> AIPSSLSINWNNYATGAYSSGNAASDFGNAGGWNQSRSYISDGTLRVTLLKNALSGAGGLISNIDVSDGTEYELDYDVRFHSQFDWSRGGKVGFGFSIGEGNTGGDPGWDGNGGTLRMMWYQTDAGRVFFQPYIYHKDQPGQY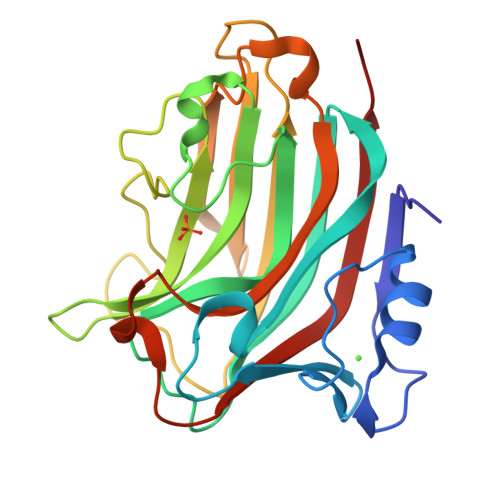GDTFGKSYPSSGSITKGTTYHVHVYIKSNTGSNRDGRAQIIINGTTVLDTAIRWTTNDAQRLIKNMTFHTFRGGSQTYWQSPVDSYIYYDNLVLRKIRLEH> GPGSEFRERYELSEKMLSACNLLKYNIKDPKALASKDMRICLNTLQHDWFRVSSQKSAVPAMVGDYIAAFEAVSPDVLRYIINMADGNGNTALHYSVFHSNFQ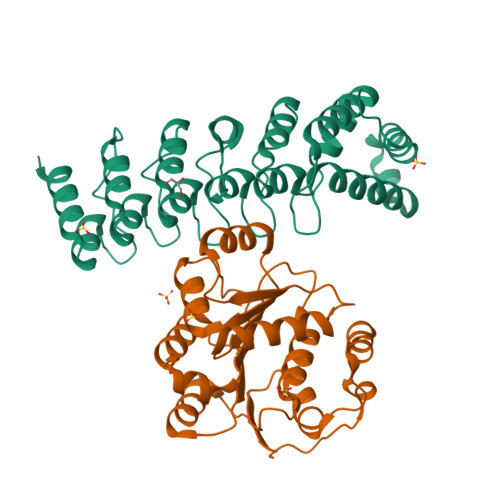IVKLLLDADVCNVDHQNKAGYTPIMLAALAAVEAEKDMQVVEELFSCGDVNAKASQAGQTALMLAVSHGRIDMVKGLLACGADVNIQDDEGSTALMCASEHGHVEIVKLLLAQPGCNGHLEDNDGSTALSIALEAGHKDIAVLLYAHLNFSKAQ;> GPGSMSASQDSRSRDNGPDGMEPEGVIESNWNEIVDSFDDMNLSESLLRGIYAYGFEKPSAIQQRAILPCIKGYDVIAQAQSGTGKTATFAISILQQIELDLKATQALVLAPTRELAQQIQKVVMALGDYMGASCHACIGGTNVRAEVQKLQMEAPHIIVGTPGRVFDMLNRRYLSPKYIKMFVLDEADEMLSRGFKDQIYDIFQKLNSNTQVVLLSATMPSDVLEVTKKFMRDPIRILVKK>GSHMSSLVRRIISTAKAPAAIGPYSQAVLVDRTIYISGQLGMDPASGQLVPGGVVEEAKQALTNIGEILKAAGCDFTNVVKATVLLADINDFSAVNDVYKQYFQSSFP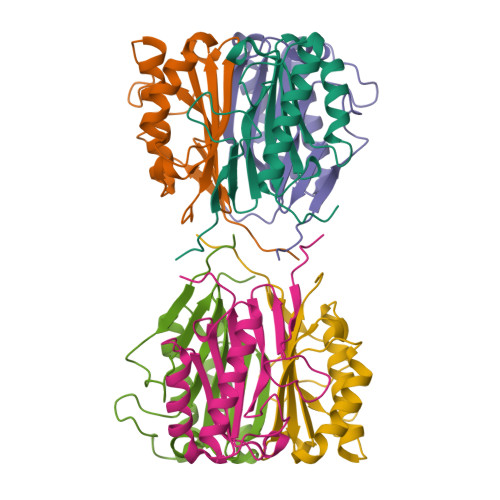AAAAYQVAALPKGGRVEIEAIAVQGPLTTASL[2x]>MRGLSRRVQAMKPDAPVAVNAKALELRRQGVDLVALTAGEPDFDTPEHVKEAARRALAQGKTKYAPPAGIPELREALAEKFRRENGLSVTPEETIVTVGGSQALFNLFQAILDPGDEVIVLSPYWVSYPEMVRFAGGVVVEVETLPEEGFVPDPERVRRAITPRTKALVVNSPNNPTGAVYPKEVLEALARLAVEHDFYLVSDEIYEHLLYEGEHFSPGRVAPEHTLTVNGAAKAFAMTGWRIGYA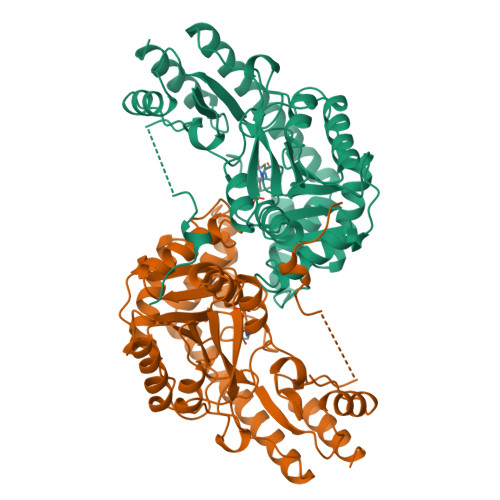CGPKEVIKAMASVSRQSTTSPDTIAQWATLEALTNQEASRAFVEMAREAYRRRRDLLLEGLTALGLKAVRPSGAFYVLMDTSPIAPDEVRAAERLLEAGVAVVPGTDFAAFGHVRLSYATSEENLRKALERFARVLGRA[4x]> ITPVN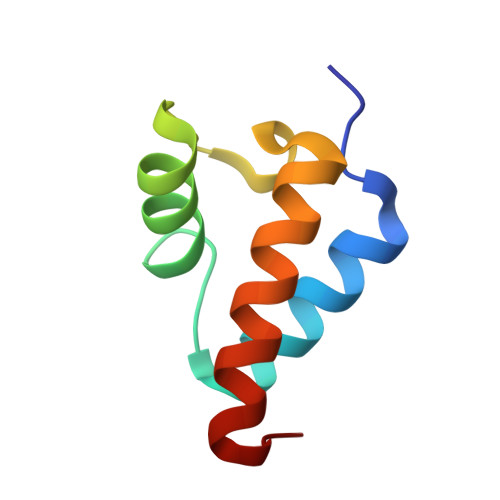DETMQEINTLLIALDKTWDDDLLPLCSQIFRRDIRASSELTQAEAVKALGFLKQKAAEQKVA>HTDLSGKVFVFPRESVTDHVNLITPLEKPLQNFTLCFRAYSDLSRAYSLFSYNTQGRDNELLVYKERVGEYSLYIGRHKVTSKVIEKFPAPVHICVSWESSSGIAEFWINGTPLVKKGLRQGYFVEAQPKIVLGQEQDS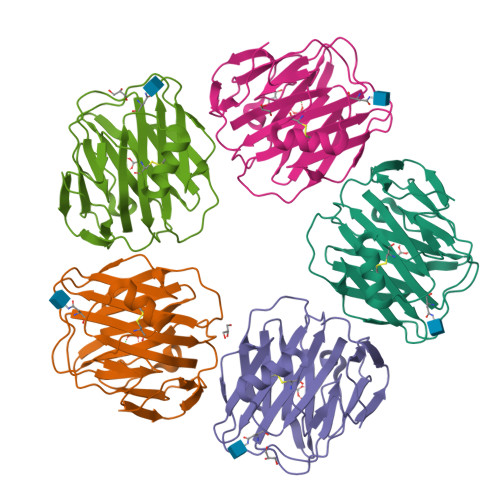YGGKFDRSQSFVGEIGDLYMWDSVLPPENILSAYQGTPLPANILDWQALNYEIRGYVIIKPLVWV[5x]> TYNITGDGNSFTPTSDMTSTAAPAIDLKPGVLNPTGKLWRPVGTSVATIDSLAIVSDRFGQYSFVNEGMRETFSKALFDINMWQPLFQATKTGCGPIVLSSFTTTTSGYVGATAGDALDNPVTNGVFISTVQIMNLQRTIAARMRDVALWQKHLDTAMTMLTPDISAGSASCNWKSLLAFAKDILPLDNLCLTYPNEFYNVAIHRYPALKPGNPDTKLPDAQAHPLGEVAGAFNAATSEVGSLVGSSSTLSQAISTMAGKDLDLIEADTPLPVSVFTPSLAPRSYRPAFIKPEDAKWIAEFNNSSLIRKTLTYSGATYTVQLGPGPTRVIDMNAMIDSVLTLDVSGTILPYDTNPDLSTSVPAFVLIQTSVPIQQVTTAANITAITVVSAAGASAINLAINVRGQPRFNMLHL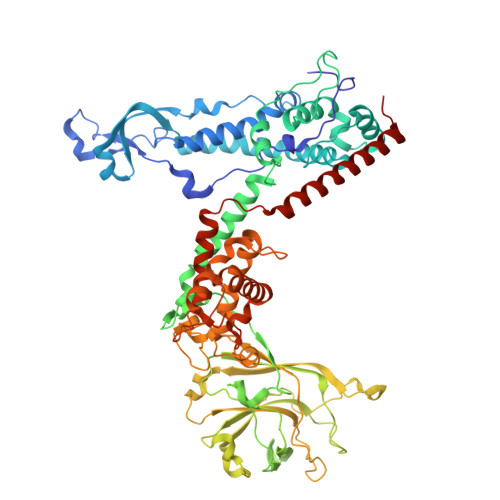QATFERETITGIPYIYGLGTFLIPSPTSSSNFSNPTLMDGLLTVTPVLLRETTYKGEVVDAIVPATVMANQTSEEVASALANDAIVLVSNHLNKLANVVGDAIPVASRTDDSATSAIVSRLAVQHKLSQVGQASPTPPDYPLLWRRAKRAASMFVSNPSLALQVGIPVLTQSGMLSALTSGVGTALRTGSLGKGVTDASEKLRARQSLTVAKQAFFDQIGSLWPGK>[2x]MFDFSKVVDRHGTWCTQWDYVADRFGTADLLPFTISDMDFATAPCIIEALNQRLMHGVFGYSRWKNDEFLAAIAHWFSTQHY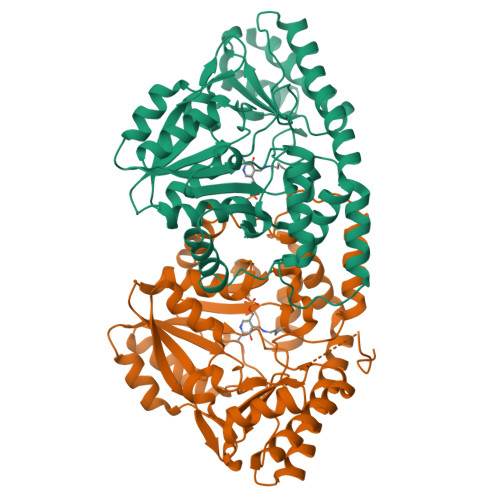TAIDSQTVVYGPSVIYMVSELIRQWSETGEGVVIHTPAYDAFYKAIEGNQRTVMPVALEKQADGWFCDMGKLEAVLAKPECKIMLLCSPQNPTGKVWTCDELEIMADLCERHGVRVISDEIHMDMVWGEQPHIPWSNVARGDWALLTSGSKSFNIPALTGAYGIIENSSSRDAYLSALKGRDGLSSPSVLALTAHIAAYQQGAPWLDALRIYLKDNLTYIADKMNAAFPELNWQIPQSTYLAWLDLRPLNIDDNALQKALIEQEKVAIMPGYTYGEEGRGFVRLNAGCPRSKLEKGVAGLINAIRAVR>[2x]GALARPCDCDVGGALDPQCDEATGQCRCRPHMIGRRCEQVQPGYFRPFLDHLTWEAEGAHGQVLEVVERLVTNRETPSWTGVGFVRLREGQEVEFLVTSLPRAMDYDLLLRWEPQVPEQWAELELVVQRPGPVSAHSPCGHVLPRDDRIQGMLHPNTRVLVFPRPVCLEPGLSYKLKLKLTGTGGRAHPETPYSGSGILIDSLVLQPHVLMLEMFSGGDAAALERRTTFERYRCHEEG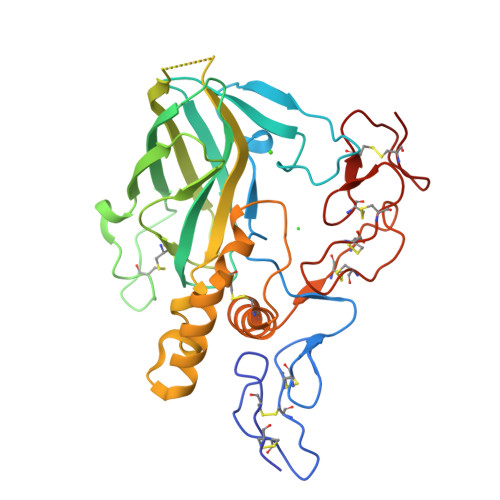LMPSKTPLSEACVPLLISASSLVYNGALPCQCDPQGSLSSECNPHGGQCRCKPGVVGRRCDACATGYYGFGPAGCQA>[2x]ASS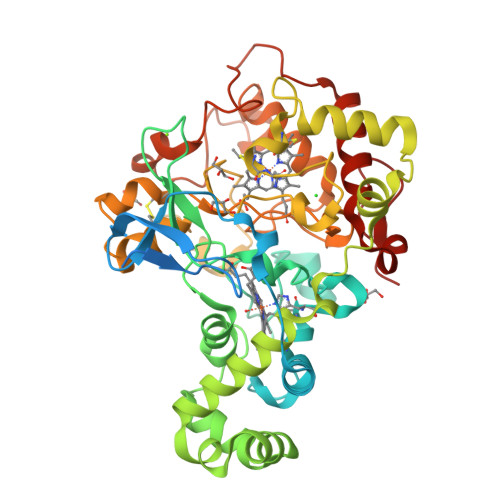GPAAPDATHSTHAARPASAASSTSPMNPTSTPGASGPAHAKAALDAARAKAAPPSPPTTVLLPGAPPERVVDTIGRGTPQVASKVDPTAAVFRPDPTLAALGKRVFFDPALSEPRGMSCASCHDPGRAFAPTLSPAALAGPRVPQGSRPGHFSRRNAPSLLYVRYVPRRHFYQDDDALAPAPFGGLFSDGRADTLAEQLRGPLFDPDEMNNASAAALMRKIGRTGLGAALAGRFGPSVRRDPERMVRVLGEAMQAYLQSDEMAPFSSRYDAYVTKRAPLTPQEMRGLALFRNPDKGNCMSCHTLSDTASRPERSLFTDFGYDAIAVPRNRALPANRDPRHFDNGLCDTAAKLRWPEPTQWCAYLRTPGLRNVAIKESFMHNGVFDTLRDAVAFMNTRSTDPARWYHGRDTFDDVPRAYRGNVNVNSTPMNRRPGTPPAMTDADVDDLVAFLRTLTDARYVGLMPTAPDGKAARP> GPTIYHAKDAVQTTKPSERKPRLVVFVVGETARADHVQFNGYGRETFPQLAKVDGLANFSQVTSCGTSTAYSVPCMFSYLGQDDYDVDTAKYQENVLDTLDRLGVGILWRDNNSDSKGVMDKLPATQYFDYKSATNNTICNTNPYNECRDVGMLVGLDDYVSANNGKDMLIMLHQMGNHGPAYFKRYDEQFAKFTPVCEGNELAKCEHQSLINAYDNALLATDDFIAKSIDWLKTHEANYDVAMLYVSDHGESLGENGVYLHGMPNAFAPKEQRAVPAFFWSNNTT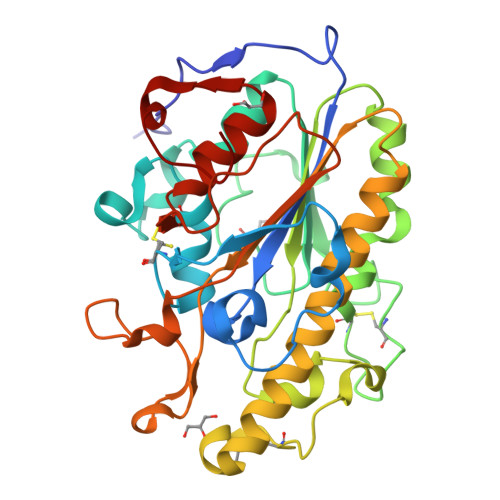FKPTASDTVLTHDAITPTLLKLFDVTAGKVKDRAAFIQ>[2x]MSNE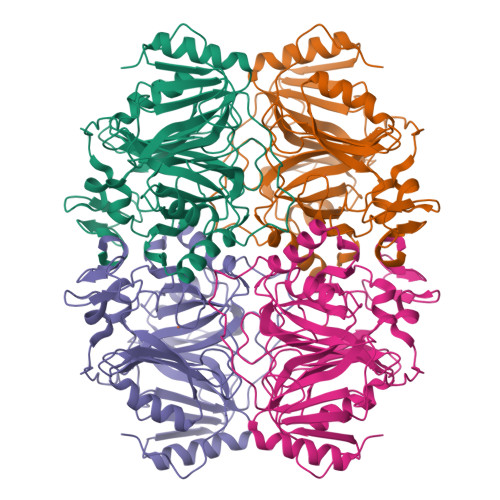IPKPVAPAPDILRCAYAELVVTDLAKSRNFYVDVLGLHVSYEDENQIYLRSFEEFIHHNLVLTKGPVAALKAMAFRVRTPEDVDKAEAYYQELGCRTERRKDGFVKGIGDALRVEDPLGFPYEFFFETTHVERLHMRYDLYSAGELVRLDHFNQVTPDVPRGRKYLEDLGFRVTEDIQDDEGTTYAAWMHRKGTVHDTALTGGNGPRLHHVAFSTHEKHNIIQICDKMGALRISDRIERGPGRHGVSNAFYLYILDPDNHRIEIYTQDYYTGDPDNPTITWNVHDNQRRDWWGNPVVPSWYTEASKVLDLDGNVQEIIERTDDSELEVTIGADGFSFTRAGDEDGSYHGQASKGFKLGNQL>[10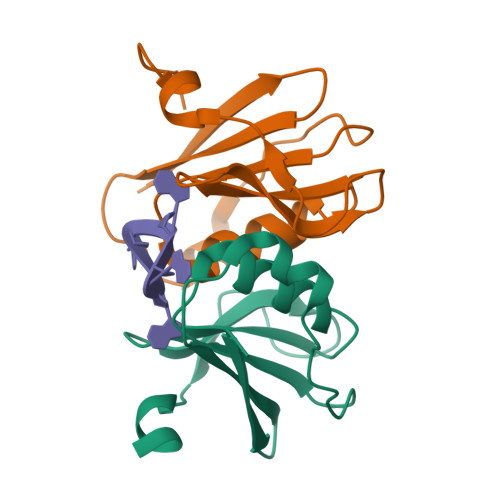x]GANAMASMKFAVIDRKNFTLIHFEIEKPIKPEILKEIEIPSVDTRKGVVISGRGPIWLHCFLAHKYAHTPFVAVYDPRLGAVVVQSHSELREGDVIDVVVEEILKGGVRHV>[2x]MKHHHHHHAMFKKVLVANRGEIACRVIRACKELGIQTVAIYNEIE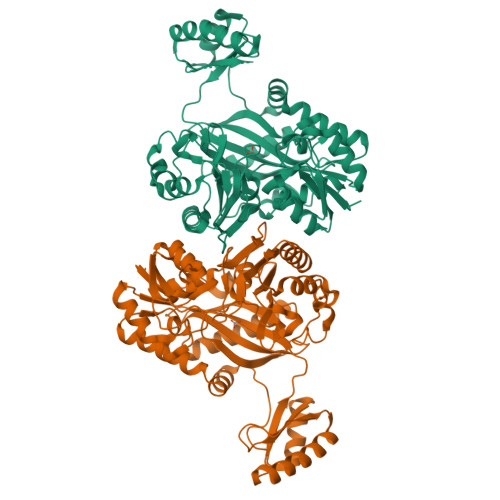STARHVKMADEAYMIGVNPLDTYLNAERIVDLALEVGAEAIHPGYGFLAENEHFARLCEEKGITFIGPHWKVIELMGDKARSKEVMKRAGVPTVPGSDGILKDVEEAKRIAKEIGYPVLLKASAGGGGRGIRICRNEEELVRNYENAYNEAVKAFGRGDLLLEKYIENPKHIEFQVLGDKYGNVIHLGERDCSIQRRNQKLVEIAPSLLLTPEQREYYGSLVVKAAKEIGYYSAGTMEFIADEKGNLYFIEMNTRIQVEHPVTEMITGVDIVKWQIRIAAGERLRYSQEDIRFNGYSIECRINAEDPKKGFAPSIGTIERYYVPGGFGIRVEHASSKGYEITPYYDSLIAKLIVWAPLWEVAVDRMRSALETYEISGVKTTIPLLINIMKDKDFRDGKFTTRYLEEHPHVFDYAEHRDKEDFVAFISAVIASYHGL> KETAAAKFERQHMDSSTSAASSSNYCNQMMKSRNLTKDRCKPVNTFVHESLADVQAVCSQKNVACKNGQTNCYQSYSTMSITDCRETGSSKYPNCAYKTTQANKHIIVACEGNPYVPVHFDASVSGSGS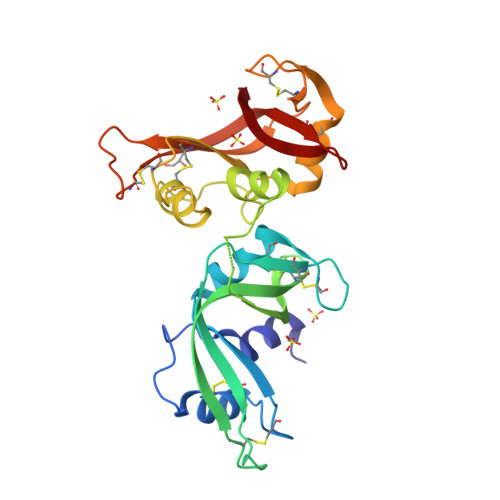GKETAAAKFERQHMDSSTSAASSSNYCNQMMKSRNLTKDRCKPVNTFVHESLADVQAVCSQKNVACKNGQTNCYQSYSTMSITDCRETGSSKYPNCAYKTTQANKHIIVACEGNPYVPVHFDASV> C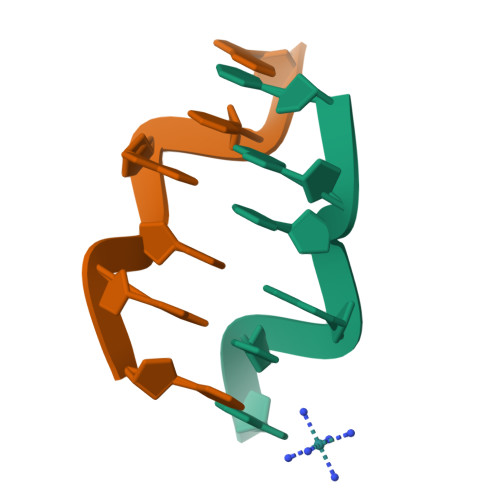GCGCA;> TGCGCG>ALLPILSFPDPRLRTIAKPVEEVTDEIRQLAADMFETMYAAPGIGLAASQVDRHIQLIVMDLSESKDEPMVFINPKVTPLTEETQPYEEGCLSVPQIYDKVDRPSRVKIEAINLEGQAFEIEADGLLAVCIQHEMDHLNGKLFVDYLSPLKRQRAREKV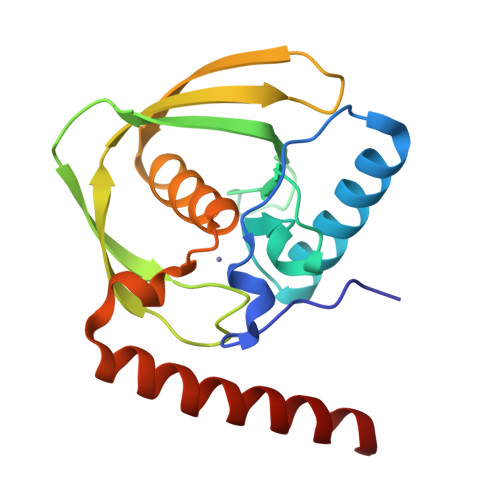EKIVRQREREKVA[2x]>GAMATSESPDAYTESFGAHTIVKPAGPPRVGQPSWNPQRASSMPVNRYRPFAEEVEPIRLRNRTWPDRVIDRAPLWCAVDLRDGNQALIDPMSPARKRRMFDLLVRMGYKEIEVGFPSASQTDFDFVREIIEQGAIPDDVTIQVLTQCRPELIERTFQACSGAPRAIVHFYNSTSILQRRVVFRANRAEVQAIATDGARKCVEQAAKYPGTQWRFEYSPESYTGTELEYAKQVCDAVGEVIAPTPERPIIFNLPATVEMTTPNVYADSIEWMSRNLANRESVILSLHPHNDRGTAVAAAELGFAAGADRIEGCLFGNGERTGNVCLVTLGLNLFSRGVDPQIDFSNIDEIRRTVEYCNQLPVHERHPYGGDLVYTAFSGSHQDAINKGLDAMKLDADAADCDVDDMLWQVPYLPIDPRDVGRTYEAVIRVNSQSGKGGVAYIMKTDHGLSLPRRLQIEFSQVIQKIAEGTAGEGGEVSPKEMWDAFAEEYLAPVRPLERIRQHVDAADDDGGTTSITATVKINGVETEISGSGNGPLAAFVHALADVGFDVAVLDYYEHAMSAGDDAQAAAYVEASVTIASPAQPGEAGRHASDPVTIASPAQPG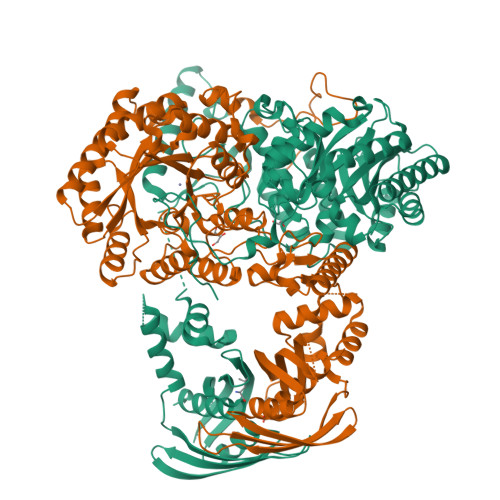EAGRHASDPVTSKTVWGVGIAPSITTASLRAVVSAVNRAAR[2x]> CGGVTPYSNESGLVNADLDV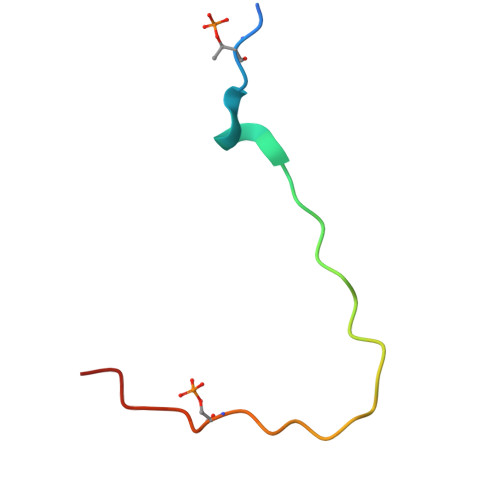KDELMFSPLVDSGS>[2x]GSHDSGDKITATSSLKTPIVNRAITESEVL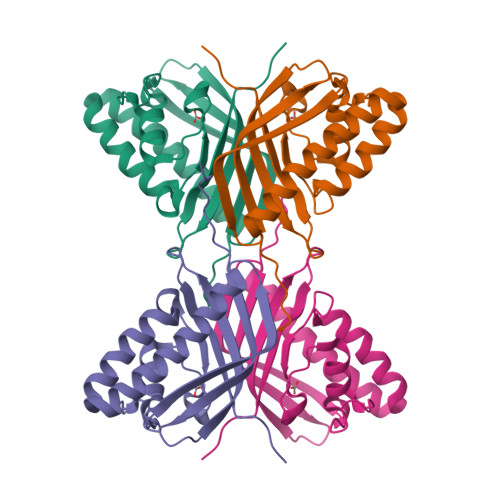AAQKAWGEALVAISTTYDAKGKASAKALAEKVIDDAYGYQFGPVLFKPTLAISPRTFRTTRAGALAYFVGDDKAFPEDKGFALSSWRKVEIKNAAIFITGNTATTMGNVIITDKQGKATTVDKTWQFLKDDHGKLRIITHHSSLPYEQ>[2x]MARKYFVAANWKCNGTLESIKSLTNSFNNLDFDPSKLDVVVFPVSVHYDHTRKLLQSKFSTGIQNVSKFGNGSYTGEVSAEIAKDLNIEYVIIGHSERRKYFHETDEDVRE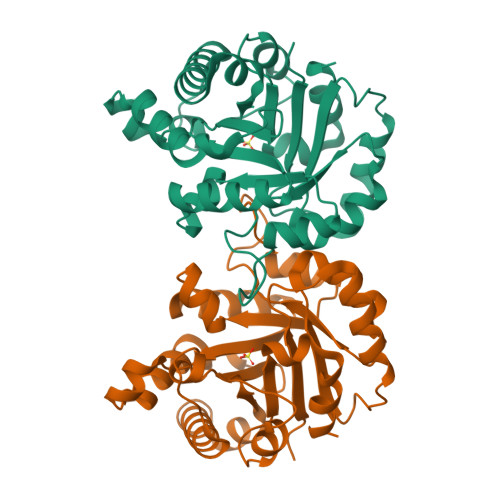KLQASLKNNLKAVVCFGESLEQREQNKTIEVITKQVKAFVDLIDNFDNVILVYEPLWAIGTGKTATPEQAQLVHKEIRKIVKDTCGEKQANQIRILYGGSVNTENCSSLIQQEDIDGFLVGNASLKESFVDIIKSAM>[2x]MMKSRTFRLSVSTLVGALVGVLMAIVGVYVTHSTEEPHTSLHEMLHDAV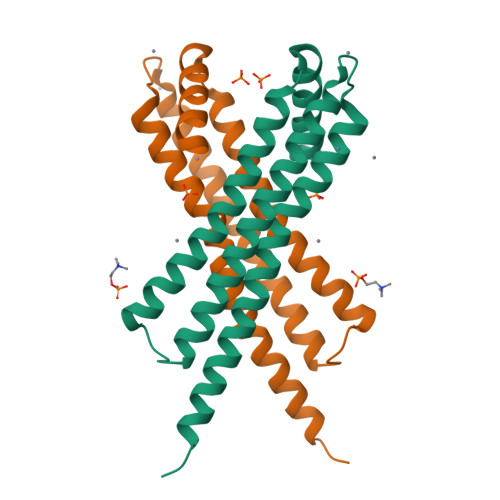PLDSNEREILELKEEEFTARRREIESRLRAANGKLAESIAKNPQWSPEVEEATREVERAAADLQRATLVHVFEMRAGLKPEHRAAYDRVLVDALKRGSQ>MTTFQELGLSQEVMKAIERMGFEETTPIQAKTIPLSLQNKDVIGQAQTGTGKTAAFGIPIVEKVDVKNGAIQALVVAPTRELAIQVSEELYKIGAVKRVRVLPIYGGQDIERQIRALKKHPHVIVGTPGRIIDHINRGTLRLEHVHTVVLDEADEMLNMGFIEDIEAILSHVPAERQTLLFSATMPDPIRRIAERFMNEPELVKVKAKEMTVPNIQQYYLEVHEKKKFDILTRLLDIQAPELAIVFGRTKRRVDELAEALNLRG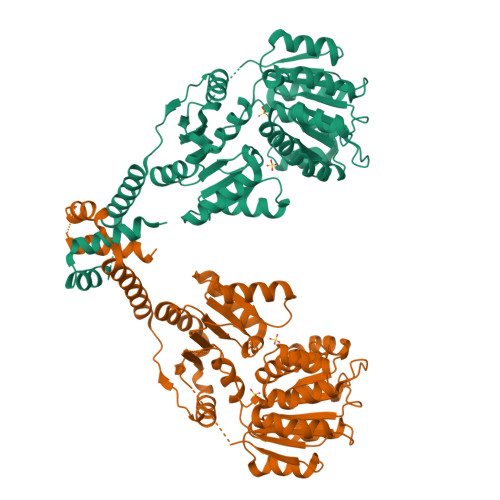YAAEGIHGDLSQAKRLSVLRKFKEGAIEILVATDVAARGLDISGVTHVYNFDIPQDPESYVHRIGRTGRAGKTGVAMTFVTPREIGQLHHIERTTKRKMERMKPPTLDEALEGQQRIAIEKLLNVVETENLSFYKRAAEELLEEHDSVTIVAACLKMLEHHHHHH[2x]The GH10 xylanase, XYL10C, from acidophilic Bispora sp. MEY-1 is an attractive candidate industrial enzyme that has remarkable activity and favorable thermostability. Among them, xylanase (endo-1,4-d-xylanase, EC 3.2.1.8) is a key enzyme that randomly cleaves the internal β-1,4-d-xylosidic linkages of xylan to yield different chain lengths of xylo-oligosaccharides. GH10 xylanases have a typical (β/α)8 barrel fold structure (also known as the typical triosephosphate isomerase barrel) with catalytic residues at the end of β-sheets 4 and 7, while GH11 xylanases display a β-jelly roll structure and employ the same retaining mechanism as GH10 xylanases. In the present study, after removal of this N-terminal sequence, the variant XYL10C-ΔN retained its hyperthermophilic characteristic but showed a 1.8- and 2.7-fold improvement in catalytic efficiency and specific activity, respectively.

To fully understand the substrate binding and catalysis mechanisms, co-crystallization of XYL10C-ΔN and xylobiose was also completed at a resolution of 1.7 Å. There is one xylobiose molecule in the open and extended active-site groove of XYL10C-ΔN, and two β-1,4-linked xylosyl moieties in subsites − 1 and − 2. Superimposition of the XYL10C-ΔN-xylobiose complex structure and the XYL10C-ΔN structure yielded a root-mean-square deviation (RMSD) value of 0.24 Å for all Cα atoms, suggesting that ligand binding did not alter the protein conformation. The xylobiose can form several hydrogen bonds, such as with Ala131, Asn132, His168, Asn218, Glu300, and Trp372 around the catalytic pocket, which provide strong binding forces to stabilize the enzyme–substrate complex and to maintain effective catalysis. Structural analysis of the XYL10C-ΔN-xylobiose complex indicated five key residues (Asn132, Lys135, His168, Asn218, and Trp372) that are involved in substrate binding via hydrogen bonds. As shown in the structure of the XYL10C-ΔN-xylobiose complex, the side chain N atom of Lys135, located on the loop 2, forms three hydrogen bonds with the hydroxyl oxygen, glycosidic oxygen, and O5 of xylobiose. These interactions limit the swing of loop 2, and further affect the interactions of the substrate and other functional amino acids. The OE2 of Glu175 shows a distance of approximately 2.9 Å to the side chain N atom of Lys135, which permits the formation of salt and hydrogen bonds. Moreover, the carboxy oxygen of Glu175 can form a hydrogen bond with the nitrogen of Met137 located on loop 2. Thus, residue Glu175 of XYL10C-ΔN, which interacts strongly to Lys135 and Met137 of loop 2, and is in close proximity to loop 3, might have the roles of stabilizing the substrate conformation in the catalytic center and affecting the catalytic efficiency of XYL10C-ΔN.

>WGLNNAARADGKLWFGTAADIPGLEQDDRYYMKEYNNTHDFGGTTPANIMKFMFTEPEQNVFNFTGAQEFLDIAFASHKLVRCHNLIWQSELPTWVTNPTTNWTNETLSKVLQNHVYTLVSHFGDQCYSWDVVNEALSDDPAGSYQNNIWFDTIGPEYVAMAFEYAEKAVKDHKLNVKLYYNDYNIEYPGPKSTAAQNIVKELKARNIQIDGVGLESHFIAGETPSQATQITNMADFTSLDIDVAVTELDVRLYLPPNATSEAQQVADYYATVAACAATERCIGITVWDFDDTYSWVPSTFAGQGYADLFFQPDGPNTPLVKKAAYDGCLQALQH[2x]Genome segregation is a fundamental process that preserves the genetic integrity of all organisms, but the mechanisms driving genome segregation in archaea remain enigmatic. This study delved into the unknown function of SegC (SSO0033), a novel protein thought to be involved in chromosome segregation in archaea. The segC (sso0033) gene encodes a 165-residue hypothetical protein of unknown function. SegC has a tertiary structure folding similar to those of the ThDP-binding fold superfamily, but SegC shares only 5–15% sequence identity with those proteins. Surprisingly, we found that SSO0033 exhibits nucleotide triphosphatase (NTPase) activity and assembles into filaments in the presence of nucleoside triphosphates (NTPs) and DNA.

After several trials, we determined the crystal structure by soaking apo-form crystal in crystallization solution with additional 20 mM ATP. From Fo – Fc ligand omit electron density map, we observed an additional electron density in the interface of the two dimers under the ATP-soaked condition, which was not observed in apo-form density map. Based on the shape and size of the electron density, we can only fit an ADP molecule. This indicated that the ATP molecule has been hydrolyzed to ADP. In this SegC-ADP complex structure, two residues (Tyr61 and Arg73) were found to interact with ADP. Residue Arg73 forms hydrogen-bond interactions with two phosphate groups, and residue Tyr61 is involved in a π–π stacking interaction with adenine. Since the ADP is positioned at the interface of the two dimers, we also identified two residues, Arg22 and Asp25, from different molecules. However, these two residues are located more than 4 Å away from ADP. The results showed that the NTPase activity of the SegC-Y61A mutant was increased 49% relative to wild-type SegC (SegC-WT), whereas that of SegC-R73A mutant was decreased by 35% compared to SegC-WT. In addition, the SegC-ADP complex has a different catalytic site compared to that of E1b-ThDP, and both Tyr61 and Arg73 are involved in SegC NTP hydrolysis activity, but neither is located in the ThDP catalysis site.

>[4x]MFEKLYSAIIYSDEFKKILLGRGVDDLEIASAYIAFLYEDLPIIGKNLCAAFLRMGLDAVYNVMPSGKVYSPRHKLYPISRYGIDGVCINCDGGKIILRISNKGYDPEDLLESKGLESRIFVSKNFKKKSMEIIEKIWDVNKIRLIARKEILERISAGGILHMIRLEHHHHHH> MENMENDENIVVGPKPFYPIEEGSAGTQLRKYMERYAKLGAIAFTNAVTGVDYSYAEYLEKSCCLGKALQNYGLVVDGRIALCSENCEEFFIPVIAGLFIGVGVAPTNEIYTLRELVHSLGISKPTIVFSSKKGLDKVITVQKTVTTIKTIVILDSKVDYRGYQCLDTFIKRNTPPGFQASSFKTVEVDRKEQVALIMNSSGSTGLPKGVQLTHENIVTRFSHARDPIYGNQVSPGTAVLTVVPFHHGFGMFTTLGYLICGFRVVMLTKFDEETFLKTLQDYKCTSVILVPTLFAILNKSELLNKYDLSNLVEIASGGAPLSKEVGEAVARRFNLPGVRQGYGLTETTSAIIITPEGDDKPGASGKVVPLFKAKVIDLDTKKSLGPNRRGEVCVKGPMLMKGYVNNPEATKELIDEEGWLHTGDIGYYDEEKHFFIVDRLKSLIKYKGYQVPPAELESVLLQHPSIFDAGVAGVPDPVAGELPGAVVVLESGKNMTEKEV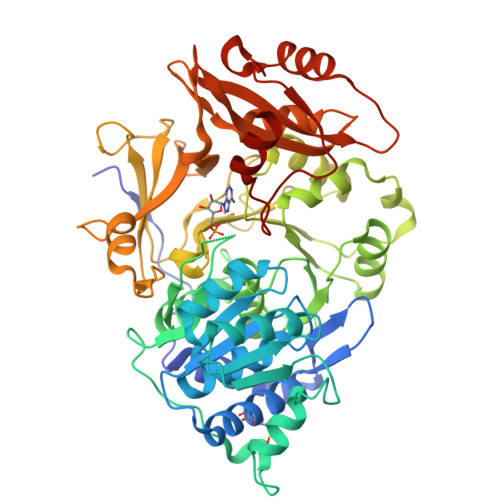MDYVASQVSNAKRLRGGVRFVDEVPKGLTGKIDGRAIREILKKPVAKM N-{[5-(dimethylamino)naphthalen-2-yl]sulfonyl}-L-alpha-glutamyl-N-[(1S)-4-{[amino(iminio)methyl]amino}-1-(chloroacetyl)butyl]glycinamide 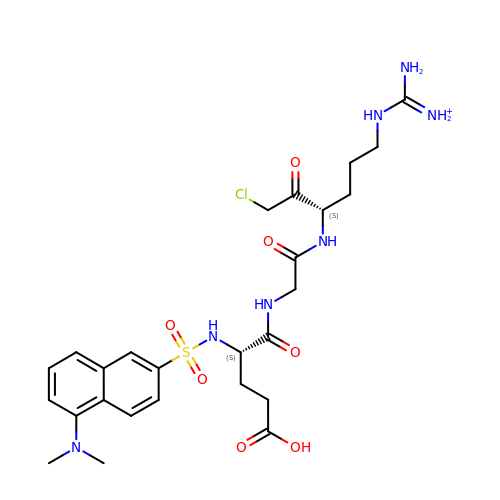| C26 H37 Cl N7 O7 S | VKQAIOBCWDJDIP-PMACEKPBSA-O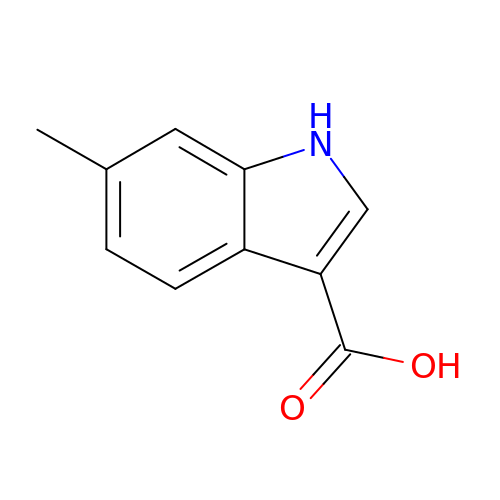6-methyl-1H-indole-3-carboxylic acid | C10 H9 N O2 | PHHZCIOPSFQASN-UHFFFAOYSA-N>[12x]SAGAGSHCQKTSLRVNFEDIGWDSWIIAPKEYEAYECKGGCFFPLADDVTPTKHAIVQTLVHLKFPTKVGKACCVPTKLSPISVLYKDDMGVPTLKYHYEGMSV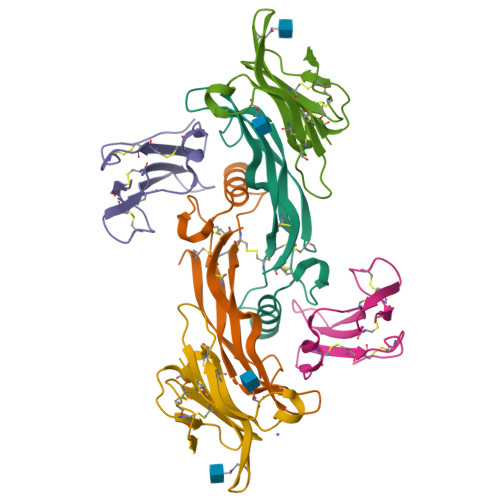AECGCR;>[12x]GADPVKPSRGPLVTCTCESPHCKGPTCRGAWCTVVLVREEGRHPQEHRGCGNLHRELCRGRPTEFVNHYCCDSHLCNHNVSLVLEATQPPSEQPGTDGQSGDDDDK;>GASGRGEAETRECIYYNANWELERTNQSGLERCEGEQDKRLHCYASWRNSSGTIELVKKGCWLDDFNCYDRQECVATEENPQVYFCCCEGNFCNERFTHLPEAGGPEVTYEPPPTAPTGDDDDK[12x]>[4x]GSHMSFRYPTDTPCTAATAAVRAGIDRDTAYGAVTPPIVLSSNFSFDGFGNKRQY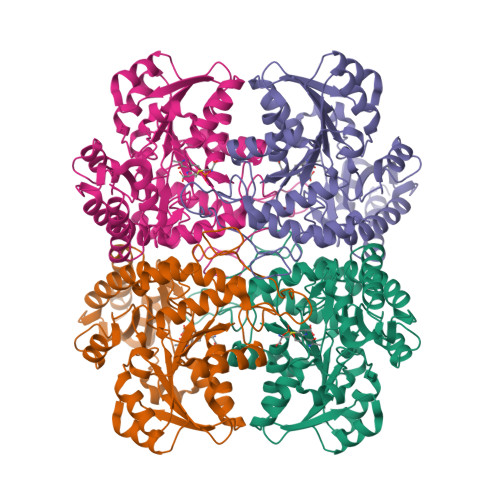DYTRSGNPTRDLLGEALAELEGGAGGVITSTGMGAINLVLNAVLQPGDTLVVPHDAYGGSWRLFNALAKKGHFALITADLTDPRSLADALAQSPKLVLIETPSNPLLRITDLRFVIEAAKKVGALTVVDNTFLSPALQKPLDFGADLVLHSTTKYINGHSDVVGGAVVARDAELHQQLVWWANALGLTGSPFDAFLTLRGLRTLDARLRVHQENADAIAELLDGHAMVNQVYFPGLATHPGHALAARQQKGFGAMMSFELEGGEAAVRAFVDGLRYFTLAESLGGVESLIAHPASMTHAAMTAEARAAAGISDGLLRLSIGIESAEDLLIDLRAGLSRAEATLTTTNRKKVDA GCN5-related N-acetyltransferase (GNAT) toxin, with an acetyltransferase activity-dependent mechanism of translation inhibition, represents a relatively new and expanding family of type II TA toxins. We here describe a group of GNAT-Xre TA modules widely distributed among Pseudomonas species. Notably, other than arresting translation through acetylating aminoacyl-tRNAs, PacT can directly bind to Fur, a key ferric uptake regulator, to attenuate its DNA-binding affinity and thus permit the expression of downstream iron-acquisition-related genes. Previously studies on GNAT-RHH TA family also observed pronounced growth arrest after expression of the GNAT-type toxin and co-expression of its upstream antitoxin gene counteracted the toxic effect. It has been also demonstrated that the translational repression function of GNAT-type toxin depend on its acetyltransferase activity which transfers the acetyl group from acetyl coenzyme A (AcCoA) to the amine group of aa-tRNAs, subsequently resulting in the inhibition of translation.

In addition, both the structures of PacT homologues from P. jinjuensis and P. flexibilis are in complex with AcCoA, and share similar fold with PacT in superposition (mean RMSD 0.28Å). Because GNAT-Xre toxins are widespread in Pseudomonas species, which also have highly conserved Fur proteins, we also tested the binding between GNAT toxins and Fur proteins from P. jinjuensis and P. flexibilis. Consistently, both PacT homologs could specifically bind to the DNA-binding domain of Fur. We also found that PacT homologs from other Pseudomonas species could bind to the Fur protein, suggesting that the direct PacT–Fur interaction is a common mechanism for PacT-type toxins. Based on these results, we conclude that the specific interactions between GNAT-Xre toxins and Fur proteins seem to be a common and novel bidirectional regulatory mechanism, indicating that Fur proteins play vital roles in bacterial iron uptake.

>MFRPLPITLQRGALRLEPMVEADVPELVELADANREVLQYMSAPQRPDWYRQAIADQREGRALPLVVRLGNRIVGTTRFLDFMPALPACEIGGTWLEQSQHGMGLNASMKYLMLRHAFDSWQMVRVQLKTAASNLRSQRAIEKLGAVREGVLRNHRRLAGGRLDDSVLYSITDHEWPQVKAALEAGFSG[4x]2-[[7-[2,6-dimethyl-4-(phenylcarbonyl)phenoxy]-1-methoxy-4-oxidanyl-isoquinolin-3-yl]carbonylamino]ethanoic 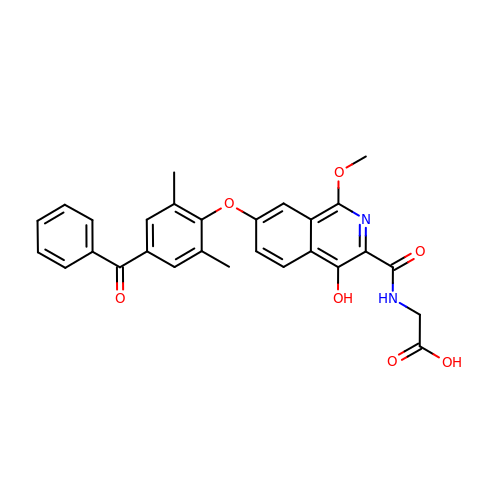acid | C28 H24 N2 O7 | ZURHRNFVXRVJAN-UHFFFAOYSA-N Stem-loop 5 (SL5, residues 150 to 294) contains the start codon of open reading frame 1a/b (ORF1a/b, residues 266 to 268). Additionally, phylogenetic covariance analysis and chemical probing experiments have shown that SL5′s secondary structure forms a four-way junction that sequesters the genome’s start codon within one of its helical stems. Beyond SARS-CoV-2, the multi-way junction and the sequestration of the start codon in a stem are conserved features across most coronaviruses, despite large sequence divergence from SARS-CoV-2 (average sequence identity of 51% for the NCBI Reference Sequences for alpha- and betacoronaviruses). SL5 has been proposed to play a role in protein–RNA or RNA–RNA binding because of its conserved hexaloops, characterized by 5′-UUYYGU-3′ (Y = C, U) repeat loop motifs.

To investigate the conservation of the SL5 fold further, we examined an additional merbecovirus ortholog, the SL5 domain of BtCoV-HKU5 (residues 188 to 320, 135 nt, 43.7 kDa). The cryo-EM structure analysis of BtCoV-HKU5 SL5 resolved four conformations (5.9, 6.4, 8.0, 7.3 Å resolution, 3.0, 3.0, 5.2, 3.0 Å modeling convergence) and again shares the same helical stacking and junction geometry with the other betacoronaviruses studied, with an inter-helical angle of 86 ± 2°. While auto-DRRAFTER was able to model all maps consistently, we deposited all these maps to EMDB but did not deposit the coordinates for conformation 3 in the PDB because the helical grooves were insufficiently resolved. As with the other three betacoronavirus domains imaged, the four-way junction is well resolved in the BtCoV-HKU5 maps, revealing a clear hole between the helical strands that separates perpendicular, coaxially stacked stems. While the four-way junction geometry is conserved between the sarbecovirus and merbecovirus orthologs, the merbecoviruses have a distinct ensemble of 3D folds that is conserved between MERS SL5 and BtCoV-HKU5 SL5. In particular, a flexible bend is observed emanating from the SL5a internal loop that allows the SL5a arm to swing in a hinge-like motion. Among these conformations, the junction geometry was conserved, with inter-helical angles occupying a narrow range of 81 to 84° and 84 to 88° for MERS and BtCoV-HKU5 SL5, respectively. Despite the junction geometry conservation, the relative locations of the hands of the SL5a and SL5b arms are variable due to the hinge in the SL5a internal loop, increasing the range of distance between UUYYGU hexaloops to 74 to 85 Å and 71 to 85 Å for MERS and BtCoV-HKU5 SL5, respectively. In addition, the merbecovirus orthologs display an unexpected tertiary interaction between the SL5a internal loop and SL5c apical loop, whereas the sarbecovirus SL5c stem is too short to form this tertiary interaction.

> GGAGCAUCGUGUCUCAAGUGCUUCACGGUCACAAUAUACCGUUUCGUCGGGUGCGUGGCAAUUCGGUGCACAUCAUGUCUUUCGUGGCUGGUGUGGCUCCUCAAGGUGCGAGGGGCAAGUAUAGAGCAGAGCUCC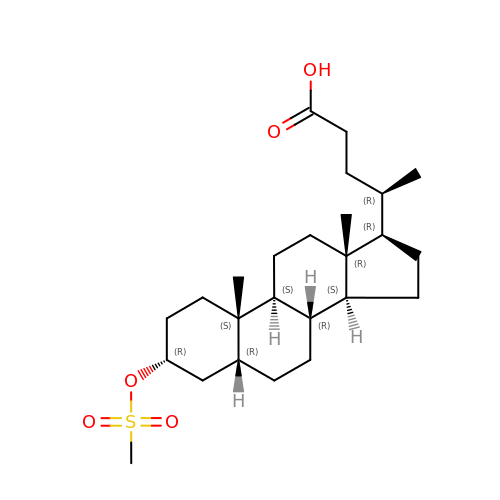(4~{R})-4-[(3~{R},5~{R},8~{R},9~{S},10~{S},13~{R},14~{S},17~{R})-10,13-dimethyl-3-methylsulfonyloxy-2,3,4,5,6,7,8,9,11,12,14,15,16,17-tetradecahydro-1~{H}-cyclopenta[a]phenanthren-17-yl]pentanoic acid | C25 H42 O5 S | QKDRPUDDQCLYDP-ULCLHEGSSA-N>SFETRFEKMDNLLRDPKSEVNSDCLLDGLDALVYDLDFPALRKNKNIDNFLSRYKDTINKIRDLRMKAEDYEVVKVIGRGAFGEVQLVRHKSTRKVYAMKLLSKFEMIKRSDSAFFWEERDIMAFANSPWVVQLFYAFQDDRYLYMVMEY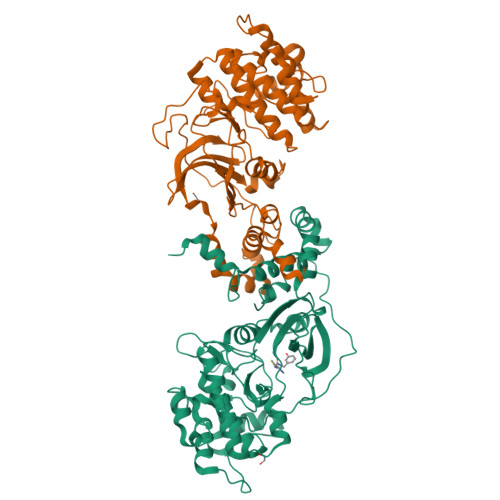MPGGDLVNLMSNYDVPEKWARFYTAEVVLALDAIHSMGFIHRDVKPDNMLLDKSGHLKLADFGTCMKMNKEGMVRCDTAVGTPDYISPEVLKSQGGDGYYGRECDWWSVGVFLYEMLVGDTPFYADSLVGTYSKIMNHKNSLTFPDDNDISKEAKNLICAFLTDREVRLGRNGVEEIKRHLFFKNDQWAWETLRDTVAPVVPDLSSDIDTSNFDDLEEDKGEEETFPIPKAFVGNQLPFVGFTYYSNRRYLSSANPNDNR[4x]Prokaryotic sodium channels, in contrast, are true tetrameric structures, composed of four identical subunits, each one equivalent to a single eukaryotic region. Both eukaryotic and prokaryotic Navs consist of voltage sensor (VS) and pore domains, which are responsible for regulation and ion-translocation functions, respectively, and C-terminal domains (CTDs), which appear in both cases to have regulatory functions, albeit of quite different natures and structures. Prokaryotic orthologues exhibit approximately 25–30% sequence identity with human Navs and several have been shown to have sodium ion translocation activity and one (NavMs from Magnetococcus marinus) has been shown to be blocked by human sodium channel blockers with similar affinities and kinetics as the human Nav1.1 isoform3, thus indicating the structure/function similarities of eukaryotic and prokaryotic Nav orthologues.

The VS is in the fully ‘activated' state, with the outward gating charge position exposed to the extracellular surface, and indeed, the activated state seen here is what would be expected at the 0 mV condition present in the crystal. The pairing of NavMs R2 and R3 with the side chain of E46, D49, and N25 in helices S2 and S1, respectively, are also clear. R1 is located at the extracellular end of S4 and is not ordered in the crystal structure. The three SF sodium ions and waters visible in the SF of this open-channel structure are virtually indistinguishable from those previously identified in the structure of the open pore-only NavMs construct13. In the NavMs channel, the pore opening is slightly narrower than in the NavMs pore (r.m.s.d. of the S6 alpha carbons∼0.4 Å), but this is still more than sufficient for the passage of at least partially-hydrated sodium ions, and much larger than the openings in any of the closed structures. The extension of the S6 helix (which is the proximal region of the CTD closest to the gate) forms an interaction motif involving specific salt bridges and hydrogen-bonded interactions with the S4–S5 linker adjacent to the intracellular surface and with Trp77 in S3. In the EEE motif (residues 229–231) near the end of the extended S6 helix, E229 forms a salt bridge with R119 in the S4–S5 linker, whilst E230 and E231 form hydrogen bonds with N238 and H237, respectively, in the top of the ‘random coil' region, leading to the C-terminal coiled-coil. R118 and Q122 in the S4–S5 linker interact (by aliphatic stacking and a hydrogen bond, respectively) with Trp77 in S3, a residue that is fully conserved among prokaryotic and human sodium channels (all isoforms and all domains) but which is not conserved in other ion channels such as potassium and TPC channels.

> GSHMSRKIRDLIESKRFQNVITAIIVLNGAVLGLLTDTTLSASSQNLLERVDQLCLTIFIVEISLKIYAYGVRGFFRSGWNLFDFVIVAIALMPAQGSLSVLRTFRIFRVMRLVSVIPTMRRVVQGMLLALPGVGSVAALLTVVFYIAAVMATNLYGATFPEWFGDLSKSLYTLFQVMTLESWSMGIVRPVMNVHPNAWVFFIPFIMLTTFTVLNLFIGIIVDAMAITKEQEEEAKTGHHQEPISQTLLHLGDRLDRIEKQLAQNNELLQRQQPQKK> TTLLNPYFGEFGGMYVPQILMPALNQLEEAFVSAQKDPEFQAQFADLLKNYAGRPTALTKCQNITAGTR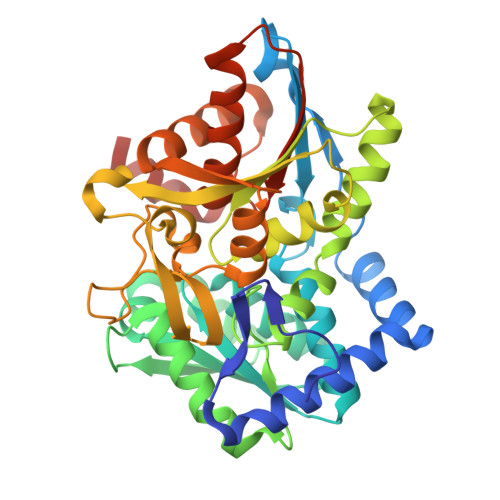TTLYLKREDLLHGGAHKTNQVLGQALLAKRMGKSEIIAETGAGQHGVASALASALLGLKCRIYMGAKDVERQSPNVFRMRLMGAEVIPVHSGSATLKDACNEALRDWPGSYETAHYMLGTAAGPHPYPTIVREFQRMIGEETKAQILDKEGRLPDAVIACVGGGSNAIGMFADFINDTSVGLIGVEPGGHGIETGEHGAPLKHGRVGIYFGMKAPMMQTADGQIEESYSISAGLDFPSVGPQHAYLNSIGRADYVSITDDEALEAFKTLCRHEGIIPALESSHALAHALKMMREQPEKEQLLVVNLSGRGDKDIFTVHDILKARGEI>MTDSIKTLSAHRSFGGVQHFHEHASREIGLPMRFAAYLPPQAEHGKVPALLYLAGLTCNEETFMVKAGAQRLAAELGIALIAPDTSPRGAHIDGESTSWDFGVGAGFYLDATAAPWAPNWRME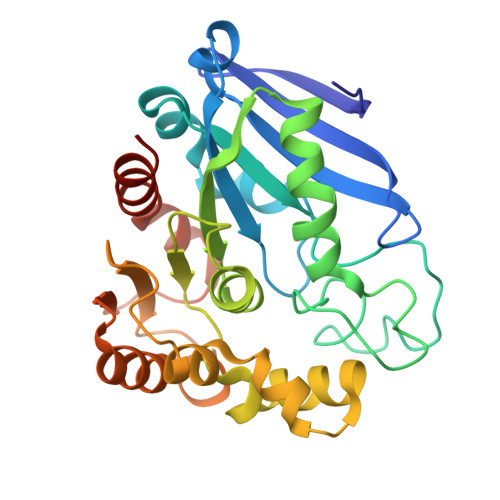SYLVDELLPLLAKTLPIDGDRIGVFGHSMGGHGALTLALRHPGLFKSLSAFAPICAPTQCPWGHKAFTGYLGADTTRWIEHDATVLMQHQPVAPYPAGILIDQGLADKFLAEQLHPHLLEDACRAIGQPLTLRRHEGYDHGYYFVQSFMADHLAHHAQILNGAIGRPAARQP[3x]> MAMPDVQYPINTYGWLK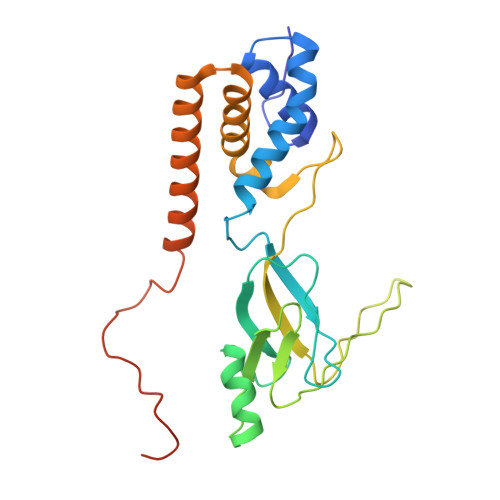KAVALWADRDDDEFVNQIPNFINFAEKEIYRNLRIPPLEKEVYLDIKDGVAYIPPDYLEAQWMMRAKDGTIFQVTSPEEISYRRQHGTINPSHWNNQPVNFARFGSRFIFYPSIEADTPYYPDDGSPLIPAENSVILSYYADPPEFHEDTDTSTILTIAPELLLYFTLRHACLFVQDDNGVQKWSALGKAILDEMVEQNKKQEYSGSPIAIPNNMTRLQSSLPDIYGIRTSRV>MKDGMRVGERFTHDFVVPPHKTVRHLYPESPEFAEFPEVFAAGFMVGLMEWACVRAMAPYLEPGEGSLGTAICVTHTAATPPGLTVTVTAELRSVEGRRLSWRVSAHDGVDEIGSGTH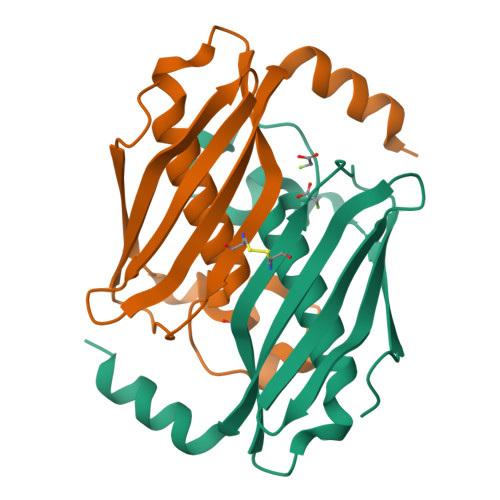ERAVIHLEKFNAKVRQKTPAG[2x]> HHHHHHSSGMGEKLELRLKSPVGAEPAVYPWPLPVYDKHHDAAHEIIETIRWVCEEIPDLKLAMENYVLIDYDTKSFESMQRLCDKYNRAIDSIHQLWKGTTQPMKLNTRPSTGLLRHILQQVYNHSVTDPEKLNNYEPFSPEVYGETSFDLVAQMIDEIKMTDDDLFVDLGSGVGQVVLQVAAATNCKHHYGVEKADIPAKYAETMDREFRKWMKWYGKKHAEYTLERGDFLSEEWRERIANTSVIFVNNFAFGPEVDHQLKERFANMKEGGRI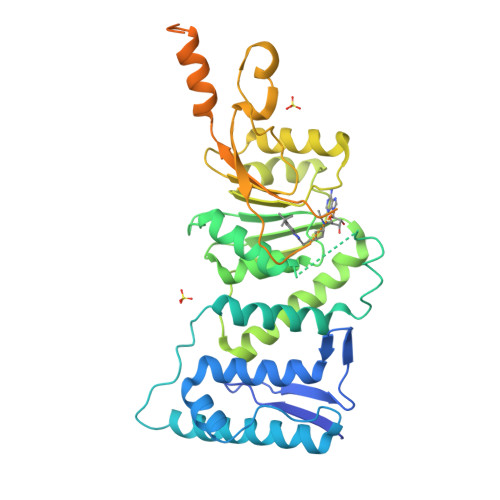VSSKPFAPLNFRINSRNLSDIGTIMRVVELSPLKGSVSWTGKPVSYYLHTIDRTILENYFSSLKNPKLREEQEAARRRQQRESKSNAATPTKGPEGKVAGPADAPMDSGAEEEKAGAATVKKPSPSKARKKKLNKKGRKMAGRKRGRPKK>MSSFVPNKEQTRTVLIFCFHLKKTAAESHRMLVEAFGEQVPTVKTCERWFQRFKSGDFDVDDKEHGKPPKRYEDAELQALLDEDDAQTQKQLAEQLEVSQQAVSNRLREMGKIQKVGRWVPHELNERQMERRKNTCEILLSRYKRKSFLHRIVTGDEKWIFFVNPKRKKSYVDPGQPATSTARPNRFGKKTMLCVWWDQSGVIYYELLKPGETVNAARYQQQLINLNRALQRKRPEYQKRQHRVIFLHDNAPSHTARAVRDTLETLNWEVLPHAAYSPDLAPSDYHLFASMGHALAE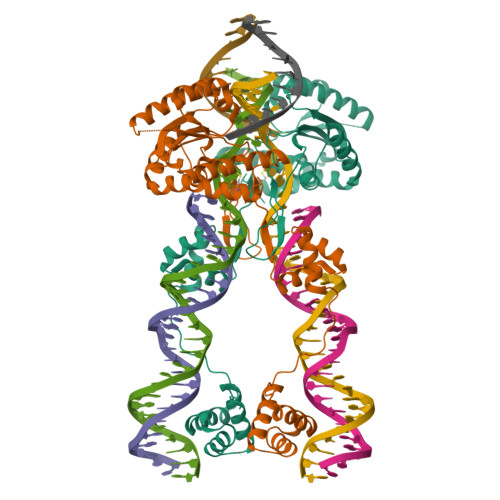QRFDSYESVKKWLDEWFAAKDDEFYWRGIHKLPERWEKCVASDGKYFE[2x]>MASPQLQMALDGFKMMGEKMAQAGGDVKAMRAVMEEMATFPSAGETKCTPVNAGGVPAEWIAAPGAADDRVILYLHGGGYVMGSITTHRETIARLSKASGARALALDYRLAPEYPFPAAVDDATAAYRWLLSQDIKPSRIVVAGDSAGGGLVLATLVALRDAKVPLPAAGVCISPWADMEGTGASMTTRAKADPVVQKEMLVNMGKTYLGGKDAKSPLAAPLHADFRGLPPLFIQVGDAETLLDDSTRVAEKAKMAGVKVDLEIWPEMPHVWHLFAPFLPEGQQAIDKIGQYVKQRTAHHHHHH[4x]

Est8 is the first member of the family of bacterial hormone‐sensitive lipases (bHSLs) for which promiscuous acyltransferase activity in water has been reported. Certain hydrolases preferentially catalyze acyl transfer over hydrolysis in an aqueous environment. Herein, we provide evidence that acyltransferase activity in esterases highly correlates with the hydrophobicity of the substrate‐binding pocket. Based on a detailed structure–function analysis of Est8 and several homologues, the present study aims to clarify molecular prerequisites for promiscuous acyltransferase activity, thereby enabling sequence‐based prediction of this remarkable phenomenon.

By screening several hydrolases using this assay, we identified a member of the family of bacterial hormone‐sensitive lipases (bHSLs), Est8, as a promiscuous acyltransferase. We observed that its substrate‐binding pocket consists of a well‐defined tunnel, which leads from the protein surface to the active site harboring a catalytic triad (Ser146, Glu240, His270). Remarkably, this tunnel is highly hydrophobic due to the presence of several methionine residues that are part of the N‐terminal cap domain, a helix‐turn‐helix motif covering the active site. As typical for bHSLs, the cap domain forms the most significant part of the substrate‐binding pocket of Est8. In contrast to the conserved C‐terminal catalytic domain, the cap domain is highly variable. As discussed for CpLIP2, CAL‐A, and MsAcT, we assumed that active‐site hydrophobicity also plays a role for the acyltransferase activity of Est8. For Est8, product hydrolysis became more dominant than acyl transfer quickly after reaching a kinetic maximum at low concentrations (ca. 27 % conversion) of 2‐phenylethyl acetate. On the way to reaching its thermodynamic equilibrium, the reaction is rapidly quenched by acidification, thus indicating high hydrolase activity. For most of them, the relative activity quickly dropped already at low alcohol concentrations, thus suggesting low stability. While Est8 and the homologues described above maintain their activity for over a month, purified WP007 precipitates within minutes after purification, resulting in a complete loss of activity. By using our hydrophobicity scoring, we were able to identify five bHSLs with much higher acyltransferase activity than Est8.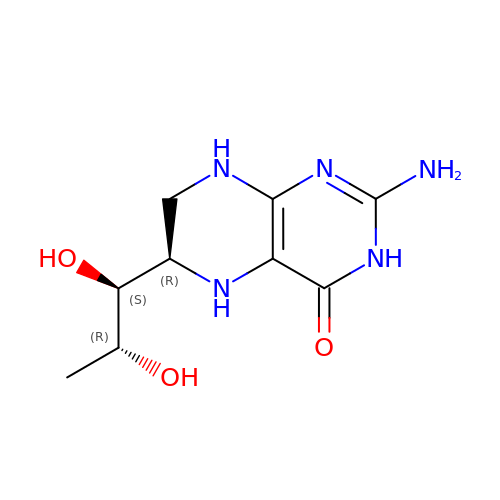6S-5,6,7,8-TETRAHYDROBIOPTERIN | C9 H15 N5 O3 | FNKQXYHWGSIFBK-ZMIZWQJLSA-N> MRGSHHHHHHTDPL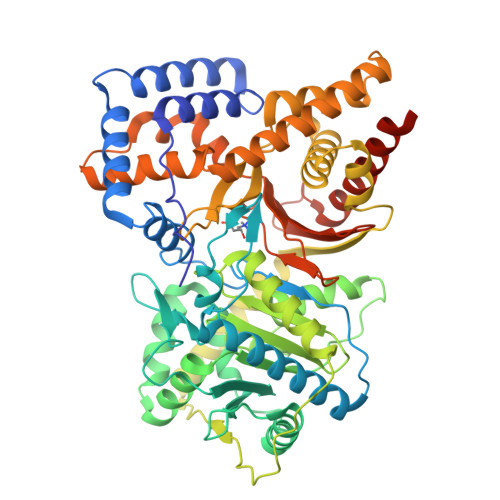PRLPVPPLQQSLDHYLKALQPIVSEEEWAHTKQLVDEFQASGGVGERLQKGLERRARKTENWLSEWWLKTAYLQYRQPVVIYSSPGVMLPKQDFVDLQGQLRFAAKLIEGVLDFKVMIDNETLPVEYLGGKPLCMNQYYQILSSCRVPGPKQDTVSNFSKTKKPPTHITVVHNYQFFELDVYHSDGTPLTADQIFVQLEKIWNSSLQTNKEPVGILTSNHRNSWAKAYNTLIKDKVNRDSVRSIQKSIFTVCLDATMPRVSEDVYRSHVAGQMLHGGGSRLNSGNRWFDKTLQFIVAEDGSCGLVYEHAAAEGPPIVTLLDYVIEYTKKPELVRSPMVPLPMPKKLRFNITPEIKSDIEKAKQNLSIMIQDLDITVMVFHHFGKDFPKSEKLSPDAFIQMALQLAYYRIYGQACATYESASLRMFHLGRTDTIRSASMDSLTFVKAMDDSSVTEHQKVELLRKAVQAHRGYTDRAIRGEAFDRHLLGLKLQAIEDLVSTPDIFMDTSYAIAMHFHLSTSQVPAKTDCVMFFGPVVPDGYGVCYNPMEAHINFSLSAYNSCAETNAARLAHYLEKALLDMRALLQSHPRAKLISEEDLSLISG> GMKLPRFGVE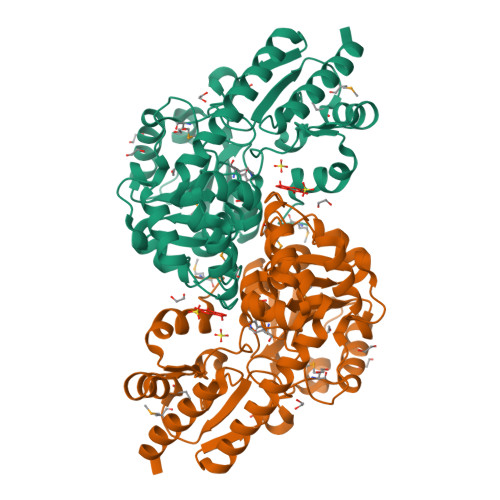EWLNVHENSAIYDIAGVSISSLTLEELFALSGTNPEDFYKKLQGTKLNYGWIEGSPAFKKSVSQLYTGVKPEQILQTNGATGANLLVLYSLIEPGDHVISLYPTYQQLYDIPKSLGAEVDLWQIEEENGWLPDLEKLRQLIRPTTKMICINNANNPTGAVMDRTYLEELVEIASEVGAYILSDEVYRSFSELDVPSIIEVYDKGIAVNSLSKTYSLPGIRIGWVAANHQVTDILRDYRDYTMICAGVFDDLVAQLALAHYQEILERNRHILEENLAILDQWIEEEPLVSYIRPAVVSTSFVKIAVDMPMEDFCLQLLQEHGVLLVPGNRFERDGYVRLGFACEQETLIKGLEKLSQFLRRFDKEN(5S)-5-{[10-(1,2,3,4-TETRAHYDROACRIDIN-9-YLAMINO)DECYL]AMINO}-5,6,7,8-TETRAHYDROQUINOLIN-2(1H)-ONE 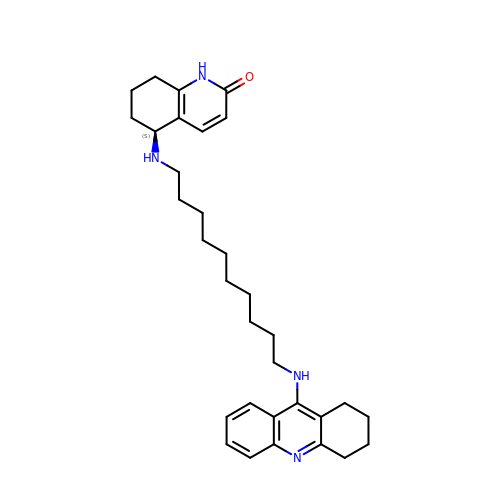| C32 H44 N4 O | ROTFGKJJMRTWBD-MHZLTWQESA-N The ferrous iron and 2-oxoglutarate (2OG)-dependent HIF prolyl hydroxylases (PHDs/EGLNs) catalyse trans-4-prolyl hydroxylations on HIFα subunits, thus promoting their binding to the von Hippel–Lindau protein (VHL), a targeting component of a ubiquitin E3 ligase, and signalling for HIFα degradation under normoxic conditions. The PHD-catalysed hydroxylations of HIF-1α/HIF-2α in higher animals occur in amino- and carboxy-terminal oxygen-dependent degradation domains (NODD and CODD). The three human PHDs exhibit different NODD/CODD selectivities, with PHD3 being substantially more selective for CODD than PHD1/2 (refs 16). Biophysical analyses employing crystallography and NMR reveal that the molecular basis of PHD isoform and variant selectivity involves enzyme–substrate interactions involving β2/β3 loop residues (that bind the LXXLAP motif) and helices α3 and α4, regions which display sequence variations between the PHD isoforms.

Using biochemical and structural studies, we identified four more residues in α3 and α3-βI loop regions (PHD2/Ile280, Arg281, Ile292 and Gly294 that are substituted in PHD3/Val102, Leu103, Val114 and Glu116, respectively) and which play roles in determining selectivity. Indeed, we found that FG2216 (IOX3)35, used in clinical trials for treatment of anaemia, preferentially displaces NODD over CODD from PHD2.

> GSHMASPNGQTKPLPALKLALEYIVPCMNKHGICVVDDFLGKETGQQIGDEVRALHDTGKFTDGQLVSQKSDSSKDIRGDKITWIEGKEPGCETIGLLMSSMDDLVLHCNGKLGSYKVNGRTKAMVACYPGNGTGYVRHVDNPNGDGRCVTCIYYLNKDWDAKVSGGILRIFPEGKAQFADIEPKFDRLLFFWSDRRNPHEVQPAYATRYAITVWYFDADERARAKVKYLTGEKGVRVELNKPSDSVGKDVF> ATITQDTPINQIFTDTALAEKMKTVLGKTNVTDTVSQTDLDQVTTLQ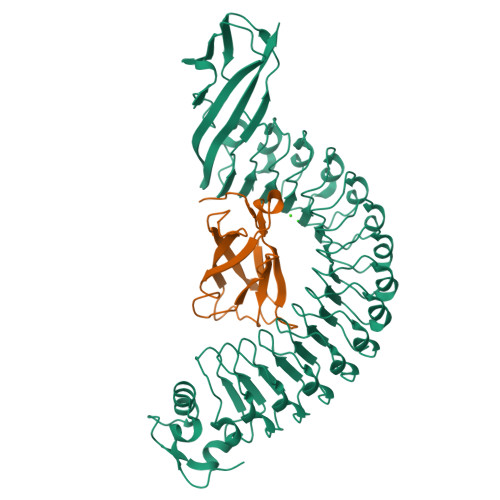ADRLGIKSIDGVEYLNNLTQINFSNNQLTDITPLKNLTKLVDILMNNNQIADITPLANLTNLTGLTLFNNQITDIDPLKNLTNLNRLELSSNTISDISALSGLTSLQQLSFSSNQVTDLKPLANLTTLERLDISSNKVSDISVLAKLTNLESLIATNNQISDITPLGILTNLDELSLNGNQLKDIGTLASLTNLTDLDLANNQISNLAPLSGLTKLTELKLGANQISNISPLAGLTALTNLELNENQLEDISPISNLKNLTYLTLYFNNISDISPVSSLTKLQRLFFSNNKVSDVSSLANLTNINWLSAGHNQISDLTPLANLTRITQLGLNDQAWTNAPVNYKANVSIPNTVKNVTGALIAPATISDGGSYTEPDITWNLPSYTNEVSYTFSQPVTIGKGTTTFSGTVTQPLKA;> GPLGSWVIPPISCPENEKGPFPKNLVQIKSNKDKEGKVFYSITGQGADTPPVGVFIIERETGWLKVTEPLDRERIATYTLFSHAVSSNGNAVEDPMEILITVTDQ> GPHMPG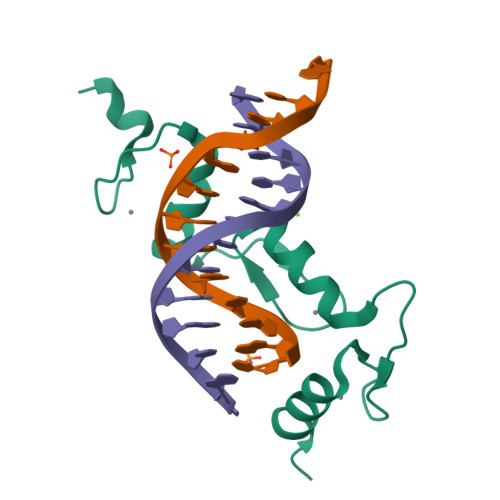RPSSKEGRRSDTCEYCGKVFKNCSNLTVHRRSHTGERPYKCELCNYACAQSSKLTRHMKTHGQVGKDVYKCEICKMPFSVYSTLEKHMKKWHSDRVLNNDIKTE> AEQKTLHIYNWTEYIAPDTVANFEKETGIKVVYDVFDSNEVLEGKLMAGSTGFDLVVPSAYFLERQLTAGVFQPLDKSKLPEWKNLDPELLK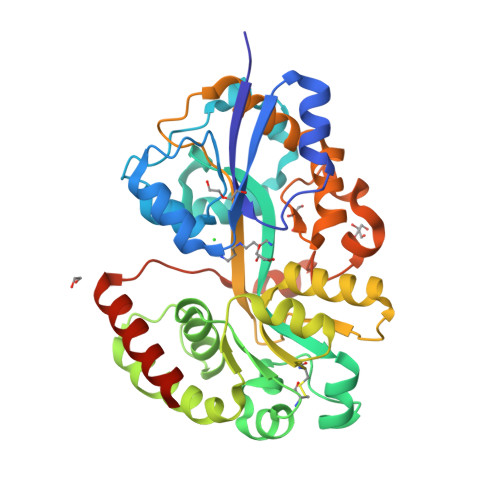LVAKHDPDNKFAMPYMWATTGIGYNVDKVKAVLGENAPVDSWDLILKPENLEKLKSCGVSFLDDPEEVFATVLNYLGKDPNSTKADDYTGPATDLLLKLRPNIRYFHSSQYINDLANGDICVAIGWAGDVWQASNRAKEAKNGVNVSFSIPKEGAMAWFDVFAMPADAKNKDEAYQFLNYLLRPDVVAHISDHVFYANANKAATPLVSAEVRENPGIYPPADVRAKLFTQKVQDPKIDRVRTRAWTKVKSGKLEHHHHHH>RSIIGGKHGDRDVRILYQVGDSEEDLPVCAPNAVCSKIDLYETPWIERQCRCPDGRTCPSSLGVEDGHTIADKTRHYKMCQPVHKLPVCKHFRDYTWTLTTAAELNVTEQIVHCRCPRNSVTYLTKREPIGNDSPGYRYLFACSPLTRLRCQRKQPCKLFTVRKRQEFLDEVNINSLCQCPKGHRCPSHHTQSGVIAGESFLEDNIQTYSGYCMANDHHHHHH[2x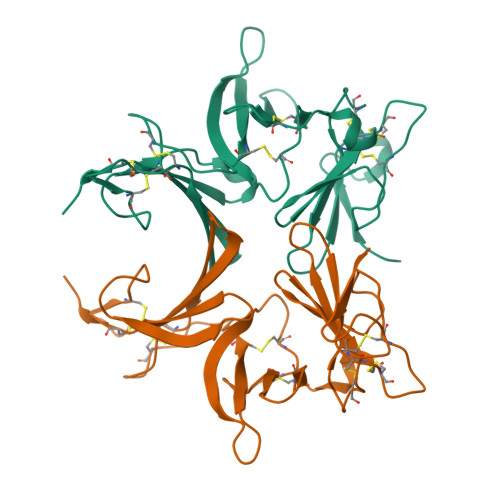]>TAPKSRNLFERNPNKELKPGENSPRQTPIFDPTVHWLFTTCGASGPHGPTQAQCNNAYQNSNLSVEVGSEGPLKGIQIWKVPATDTYSISGYGAAGGKGGKNTMMRSHGVSVLGIFNLEKDDMLYILVGQQGEDACPSTNQLIQKVCIGENNVIEEEIRVNRSVHEWAGGGGGGGGATYVFKMKDGVPVPLIIAAGGGGRAYGAKTDTFHPERLENNSSVLGLNGNSGAAGGGGGWNDNTSLLWAGKSLQEGATGGHSCPQAMKKWGWETRGGFGGGGGGCSSGGGGGGYIGGNAASNNDPEMDGEDGVSFISPLGILYTPALK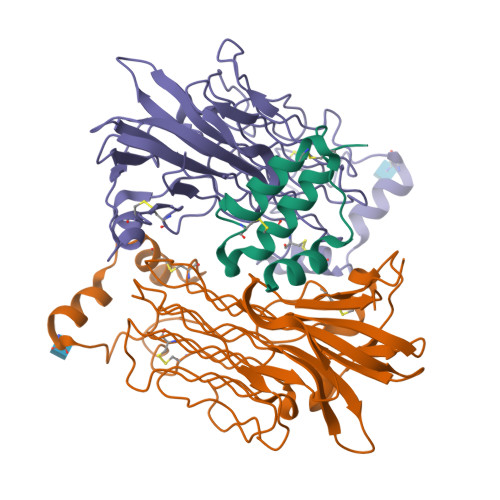VMEGHGEVNIKHYLGTDEVD[4x];>PSPEQRVEIVPRDLRMKDKFLKHLTGPLYFSPKCSKHFHRLYHNTRDCTIPAYYKRCARLLTRLAVSPVCMEDKQGTDEVD[2x]> GDRVADVIESSIGDSVSRALTRALPAPTGQDTQVSSHRLDTGKVPALQAAEIGASSNASDESMIETRCVLNSHSTAETTLDSFFSRAGLVGEIDLPLEGTTNPNGYANWDIDITGYAQMRRKVELFTYMRFDAEFTFVACTPTGQVVPQLLQYMFVPPGAPEPDSRESLAWQTATNPSVFVKLSDPPAQVSVPFMSPASAYQWFYDGYPTFGEHKQEKDLEYGACPNNMMGTFSVRTVGTSKSKYPLVIRIYMRMKHVRAWIPRPMRNQNYLFKANPNYAGNFIKPTGASRTAITTL;> SPSAEACGYSDRVAQLTIGNSTITTQEAANIIVGYGEWPSYCSDSDATAVDKPTRPDVSVNRFYTLDTKLWEKSSKGWYWKFPDVLTETGVFGQNAQFHYLYRSGFCIHVQCNASKFHQGALLVAVLPEYVIGSVAGGTGTEDTHPPYKQTQPGADGFELQHPYVLDAGIPISQLTVCPHQWINLRTNNCATIIVPYINALPFDSALNHCNFGLLVVPISPLDYDQGATPVIPITITLAPMCSEFAGLRQAVTQ;> GFPTELKPGTNQFLTTDDGVSAPILPNFHPTPCIHIPGEVRNLLELCQVETILEVNNVPTNATSLMERLRFPVSAQAGKGELCAVFRADPGRSGPWQSTLLGQLCGYYTQWSGSLEVTFMFTGSFMATGKMLIAYTPPGGPLPKDRATAMLGTHVIWDFGLQSSVTLVIPWISNTHYRAHARDGVFDYYTTGLVSIWYQTNYVVPIGAPNTAYIIALAAAQKNFTMKLCKDASDILQTGTIQ;> MGSQVSTQRSGSHENSNSATEGSTINYTTINYYKDSYAATAGKQSLKQDPDKFANPVKDIFTEMAAPLK

Enteroviruses particles are composed of single-strand RNA (virion RNA) genomes encapsulated by an icosahedral capsid of ~30 nm in diameter. In this study, we genetically perturb this equilibrium in a non-enveloped virus, enterovirus A71 to determine its structural basis. We isolate a single-point mutation variant with increased particle thermotolerance and decreased efficiency of cell entry. Using cryo-electron microscopy and molecular dynamics simulations, we determine that the thermostable native particles have acquired an expanded conformation that results in a significant increase in protein dynamics.

The single VP1 mutation of lysine 162 to glutamic acid drastically altered the structure of the native capsid. The particle was reconstructed to a resolution of 4.2 Å. Strikingly, the K162E particle was larger and resembled an A-particle conformation of the WT particle. The thermostable K162E capsid had expanded from 300–330 Å in diameter. The expansion of the K162E global capsid can be attributed to both the enlarged capsid protein shell and the increased volume of the internal cavity, which accommodated the virion RNA. The K162E particle maintained key structural elements in the WT structure, where the jelly-roll beta-barrel central core is nearly identical to that of WT. The analysis of the Coulomb potential map reveals that the 162 containing-loops have rotated. In addition, the side chain undergoes a rotation towards the core of the VP1 beta-barrel (compare Fig. 4g, f). As well, a hydrogen bond may form between the new glutamic acid 162 and asparagine 108. Although the resolution is insufficient for robust conclusions, the Coulomb potential suggests a potential new conformation in the VP1 GH loop (residues 204–224) and VP2 EF loop, which could modify the exit of the pocket factor.1-(beta-D-ribofuranosyl)-2-thioxo-2,3-dihydropyrimidin-4(1H)-one | C9 H12 N2 O5 S | 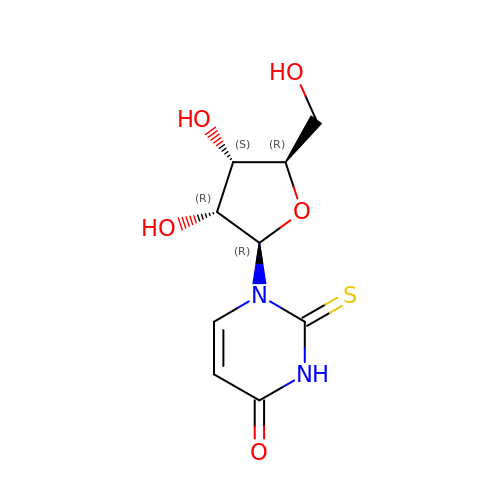GJTBSTBJLVYKAU-XVFCMESISA-N N-myristoyltransferase (NMT) is an essential eukaryotic enzyme and a validated drug target for combating malaria. N-myristoyltransferase (NMT) is an essential enzyme in eukaryotes that catalyzes the transfer of myristate from myristoyl-coenzyme A (myrCoA) to the N-terminal glycine residue of a nascent polypeptide at the ribosome. Protein myristoylation generally aids in membrane localization as well as protein-protein interactions and stability by increasing the protein’s hydrophobicity. Although multiple Plasmodium NMT inhibitors have been identified, achieving high selectivity against human NMTs remains a major challenge because of the high degree of sequence homology between human and Plasmodium peptide binding sites, where all known inhibitors bind.

We determined the X-ray co-crystal structure of PvNMT, myrCoA, and 12b at 1.65 Å resolution. Comparison with the structure of inhibitor-free PvNMT shows that conformational changes occur throughout much of the substrate binding sites. The inhibitor binding site architecture is unique relative to those of all crystal structures of PvNMT and HsNMT1 thus far characterized, with Tyr211, His213, Phe226, and Leu410 displaying distinct conformations. Compound 12b aligns closely with that of IMP-1002, reflecting the similarity of their chemical topologies, and its piperazine group binds in a similar location to that of DDD85646. As a result, N4 makes weaker electrostatic interactions with the C-terminal carboxylate group (separation distance of 4.0 Å) but is positioned more closely to Thr197, forming a hydrogen bond with the side chain hydroxyl group. Additionally, the core group stabilizes a highly rotated conformation of Tyr211, which is also observed in the IMP-1002-bound structure of PvNMT and proposed to represent a selective (S) state. The nitrogen atom of the pyridine ring of 12b forms a hydrogen bond with an additional water molecule accommodated in this region of the binding site relative to that of IMP-1002. This difference, together with the misalignment of the piperazine with Leu410, is associated with an orientational change in the inhibitor and displacement of Tyr211. The high selectivity is likely attributed to the distinct way the core and head groups interface with the adjacent waters and polar sites near the carboxy terminus, which accompanies conformational changes that propagate throughout the peptide and myrCoA binding sites.

> GPDYKFWYTQPVPKINDEFNESVNEPFISDNKVEDVRKDEYKLPPGYSWYVCDVKDEKDRSEIYTLLTDNYVEDDDNIFRFNYSAEFLLWALTSPNYLKTWHIGVKYDASNKLIGFISAIPTDICIHKRTIKMAEVNFLCVHKTLRSKRLAPVLIKEITRRINLENIWQAIYTAGVYLPKPVSDARYYHRSINVKKLIEIGFSSLNSRLTMSRAIKLYRVEDTLNIKNMRLMKKKDVEGVHKLLGSYLEQFNLYAVFTKEEIAHWFLPIENVIYTYVNEENGKIKDMISFYSLPSQILGNDKYSTLNAAYSFYNVTTTATFKQLMQDAILLAKRNNFDVFNALEVMQNKSVFEDLKFGEGDGSLKYYLYNWKCASFAPAHVGIVLL(1S,2R)-1,2-bis(3-methoxy-4-oxidanyl-phenyl)propane-1,3-diol 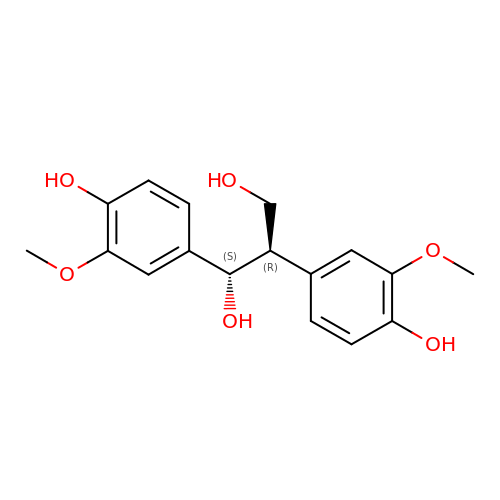| C17 H20 O6 | DFUOJBWSSSODTR-YVEFUNNKSA-N>MVSTRETVNELLRRIAAGDPGRIAELYAEEVSWKLSWPAGDHMGVVPWIQQRSTRAGVEEHFRLIADHHVAKQ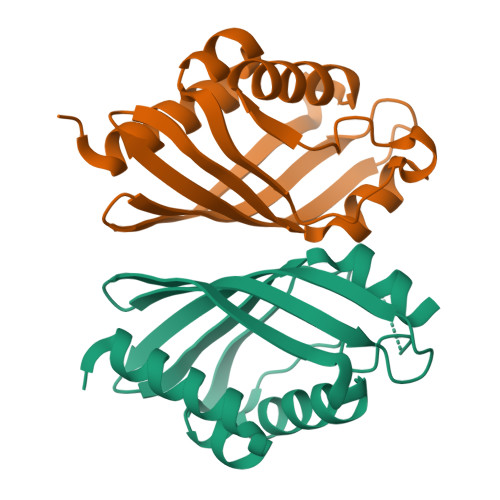SSAEVFSVLVDGADAVVLGELRNTAGPTGRSYEAPFALHLTVENGLVTRHHVYEDSLAVFRAFAENAGEPVRSRAS[2x]>[2x]AALTEKTDIFESGRNGKPNKDGIKSYRIPALLKTDKGTLIAGADERRLHSSDWGDIGMVIRRSEDNGKTWGDRVTITNLRDNPKASDPSIGSPVNIDMVLVQDPETKRIFSIYDMFPEGKGIFGMSSQKEEAYKKIDGKTYQILYREGEKGAYTIRENGTVYTPDGKATDYRVVVDPVKPAYSDKGDLYKGNQLLGNIYFTTNKTSPFRIAKDSYLWMSYSDDDGKTWSAPQDITPMVKADWMKFLGVGPGTGIVLRNGPHKGRILIPVYTTNNVSHLNGSQSSRIIYSDDHGKTWHAGEAVNDNRQVDGQKIHSSTMNNRRAQNTESTVVQLNNGDVKLFMRGLTGDLQVATSKDGGVTWEKDIKRYPQVKDVYVQMSAIHTMHEGKEYIILSNAGGPKRENGMVHLARVEENGELTWLKHNPIQKGEFAYNSLQELGNGEYGILYEHTEKGQNAYTLSFRKFNWDFLSK

Streptococcus pneumoniae genomes encode three sialidases, NanA, NanB and NanC, which are key virulence factors that remove sialic acids from various glycoconjugates. Sialidases are one key virulence factor as they remove sialic acid from host cell-surface glycans, probably unmasking certain receptors to facilitate bacterial adherence and colonization. The 115 kDa NanA is the largest of the three sialidases and is anchored to the bacterial membrane. Although recombinantly expressed full-length NanA was soluble, it failed to crystallize; therefore, a 56.5 kDa domain that retained full enzyme activity was subcloned.

The purified enzyme was crystallized in 0.1 M MES pH 6.5, 30%(w/v) PEG 4000 using the sitting-drop vapour-diffusion method. The structure of CNanA shows the canonical six-bladed β-propeller fold common to all sialidases. CNanA and NanI share 41% sequence identity and the r.m.s.d. between 413 Cα atoms is 1.26 Å. The two monomers in the asymmetric unit are related by a noncrystallographic twofold axis, superimpose with an r.m.s.d. of 0.39 Å over 470 Cα atoms and bury ∼1200 Å2 of surface at their dimer interface. The calibrated gel filtration suggests that CNanA is predominantly a monomer in solution; however, it is possible that full-length NanA may be a dimer on the bacterial surface. The active site contains the usual catalytic residues common to all sialidases: three arginines (Arg347, Arg663, Arg721) that interact with the carboxylate group of sialic acid, a nucleophilic tyrosine (Tyr752) that is proposed to form a covalent intermediate and its associated glutamic acid (Glu647), an aspartic acid (Asp372) that acts as an acid/base and a hydrophobic pocket that accommodates the acetamidomethyl group of sialic acid.>[2x]ELYTQYNRVWIPDPEEVWKSAEIAKDYRVGDKVLRLLLEDGTELDYSVNPESLPPLRNPDILVGENDLTALSYLHEPAVLHNLRIRFAESKLIYTYSGIILVAMNPYKQLPIYGDAIIHAYSGQNMGDMDPHIFAVAEEAYKQMARNNRNQSIIVSGESGAGKTVSARYAMRYFATVSKSGSNAHVEDKVLASNPITEAVGNAKTTRNDNSSRFGKYTEISFDEQNQIIGANMSTYLLEKSRVVFQSENERNYHIFYQLCASAQQSEFKHLKLGSAEEFNYTRMGGNTVIEGVNDRAEMVETQKTFTLLGFKEDFQMDVFKILAAILHLGNVQITAVGNERSSVSEDDSHLKVFCELLGLESGRVAQWLCNRKIVTSSETVVKPMTRPQAVNARDALAKKIYAHLFDFIVERINQALQFSGKQHTFIGVL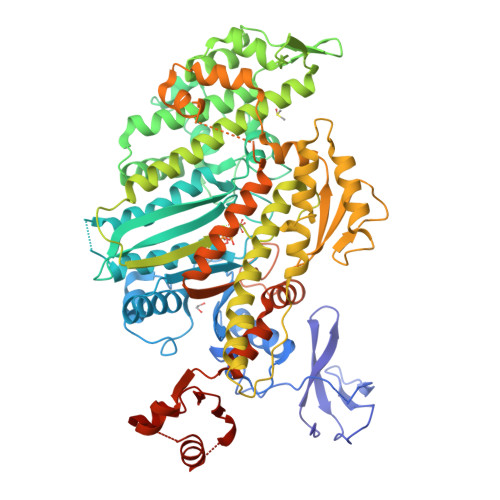DIYGFETFDVNSFEQFCINYANEKLQQQFNMHVFKLEQEEYMKEDIPWTLIDFYDNQPVIDLIEAKMGILELLDEECLLPHGTDENWLQKLYNNFVNRNPLFEKPRMSNTSFVIQHFADKVEYKCEGFLEKNRDTVYDMLVEILRASKFHLCANFFQENPTPPSPFGSMITVKSAKQVIKPNSKHFRTTVGSKFRSSLYLLMETLNATTPHYVRCIKPNDEKLPFEFDSKRIVQQLRACGVLETIRISAQSYPSRWTYIEFYSRYGILMTKQELSFSDKKEVCKVVLHRLIQDSNQYQFGKTKIFFRAGQVAYLEKLRLD> MDEKLLKTIAESKYLVALTGAGVSAESGIPTFRGKDGLWNRYRPEELANPQAFAKDPEKVWKWYAWRMEKVFNAQPNKANQAFAELERLGVLKCLITQNVDDLHERAGSRNVIHLHGSLRVVRCTSCNNSFEVESAPKIPPLPKCDKCGSLLRPGVVWFGEMLPPDVLDRAMREVERADVIIVAGTSAVVQPAASLPLIVKQRGGAIIEINPDETPLTPIADYSLR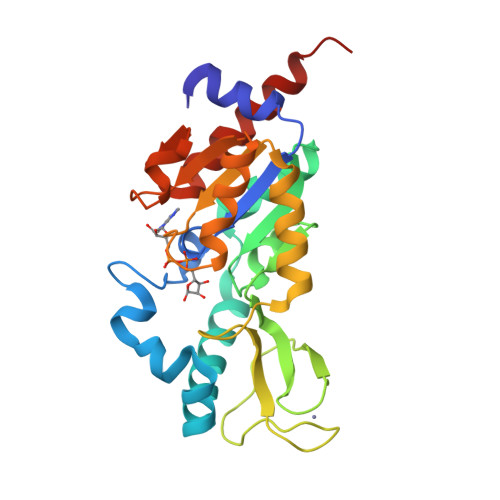GKAGEVMDELVRHVRKALSLKLN> MEATLGSGNLRQ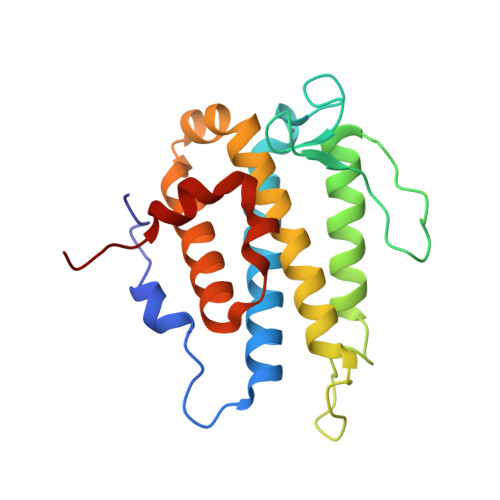AVMLPEGEDLNEWIAVNTVDFFNQINMLYGTITEFCTEASCPVMSAGPRYEYHWADGTNIKKPIKCSAPKYIDYLMTWVQDQLDDETLFPSKIGVPFPKNFMSVAKTILKRLFRVYAHIYHQHFDSVMQLQEEAHLNTSFKHFIFFVQEFNLIDRRELAPLQELIEKLGSKDR> SNAYNLQMDIPHAPTVVLTVQDLEQMEATQYTTMLPWLSAPATFTGVKLSTLLSQQYGFIPNRVTLR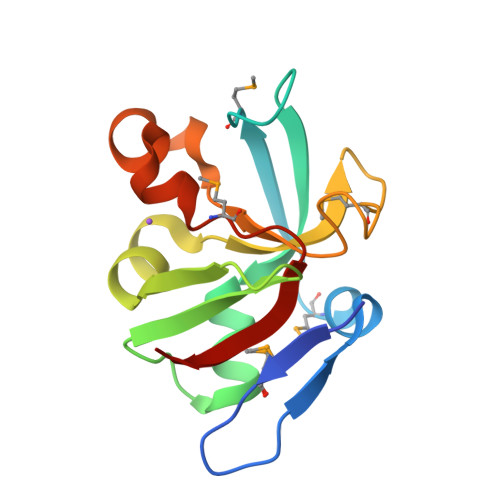ALNDYAADIDLSDIEKYQPIVAYRQDGKPMRVRDKGPFWLIYPQSSFPKELNNERYHSQMVWQLKQIHIAK> MGSSHHHHHHSSGHIEGRHDQNFYSLLGVSKTASSREIRQAFKKLALKLHPDKNPNNPNAHGDFLKINRAYEVLKDEDLRKKYDKYGEKGLEDNQGGQYESWSYYRYDFGIYDDDPEIITLERREFDAAVNSGELWFVNFYSPGSSHSHDLAPTWREFAKEVDGLLRIGAVNCGDDRMLCRMKGVNSYPSLFIFRSGMAAVKYNGDRSKESLVAFAMQHVRSTVTELSTGNFVNAIETAFAAGVGWLITFCSKGEDCLTSQTRLRLSGMLDGLVNVGWVDCDAQDSLCKSLDTTASTTAYFPPG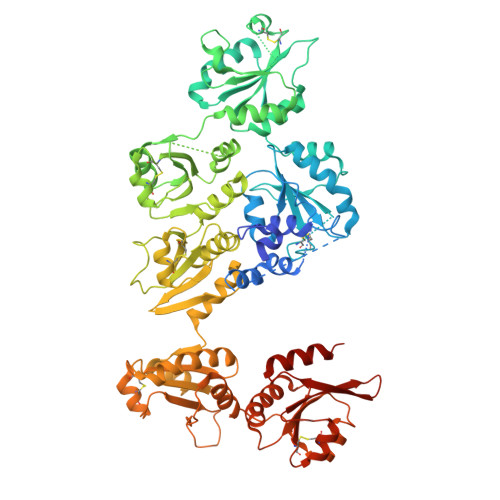ATLNDREKSSVLFLNSLDAKEIYMEIIHNLPDFELLSANQLEDRLAHHRWLVFFHFGKNENANDPELKKLKTLLKNEHIQVVRFDCSSAPGICSDLYVFQPSLAVFKGQGTKEYEIHHGKKILYDILAFAKESVNSHVTTLGPQNFPASDKEPWLVDFFAPWSPPSRALLPELRKASTLLYGQLKVGTLDCTIHEGLCNMYNIQAYPTTVVFNQSSIHEYEGHHSAEQILEFIEDLRNPSVVSLTPSTFNELVKQRKHDEVWMVDFYSPWSHPSQVLMPEWKRMARTLTGLINVGSVDCGQYHSFCTQENVQRYPEIRFYPQKSSKAYQYHSYNGWNRDAYSLRSWGLGFLPQASIDLTPQTFNEKVLQGKTHWVVDFYAPWSGPSQNFAPEFELLARMIKGKVRAGKVDCQAYPQTCQKAGIKAYPSVKLYQYERAKKSIWEEQINSRDAKTIAALIYGKLETLQSQVKRNKDEL6-[1,1-bis(oxidanylidene)-1,4-thiazinan-4-yl]-4-[[4-[4-chloranyl-3-(trifluoromethyl)phenoxy]-3,5-bis(fluoranyl)phenyl]methoxy]-1-methyl-pyrimidin-2-one 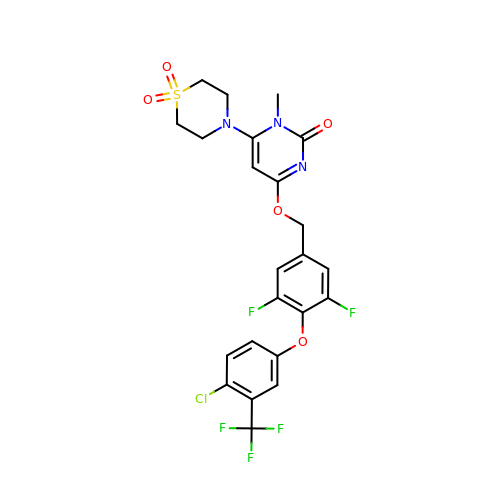| C23 H19 Cl F5 N3 O5 S | FLCSHCSBIFPQJJ-UHFFFAOYSA-N> METTEVIEGKNITVERTGEENRRLIFQDCLCAVCGLCGEICPVSAIEVNPTGAMVRTEQEKSKIAIDENKCVLCGMCSSICPFQALDLQIDGTSIKELAEYPKIIKSAEIDDETCIQCKACETACPQDAITITRELPERKDLVTGEIEIDKDTCIYCGMCEEMCPVDAIEIDHQTPSSASPVVATDIRVDEDKCVHCGICKRICPVDAIMQVCRICPYGEYEIKTPEVTGTSYIDPELCVNCGWCQEICPVDAATVTKPFEGELIIDQDTCQACETCVMVCPCNVL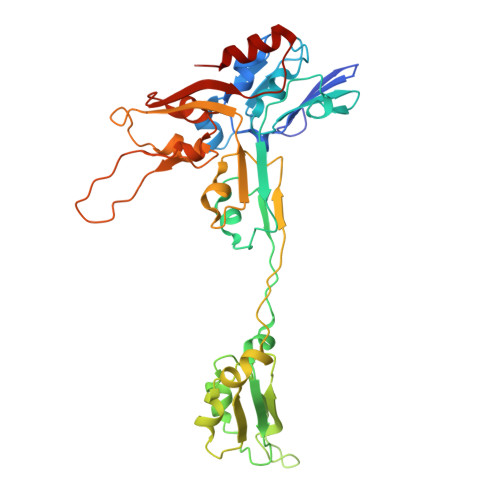SFPKPEKPGEKTTKLHKDERFCIYCGACERSCPVTAITVKRNRINTTPIRSKAWKNAFDSLLK>MPFVKGFEPISLRDTNLFEPIKIGNTQLAHRAVMPPLTRMRATHPGNIPNKEWAAVYYGQRAQRPGTMIITEGTFISPQAGGYDNAPGIWSDEQVAEWKNIFLAIHDCQSFAWVQLWSLGWASFPDVLARDGLRYDCASDRVYMNATLQEKAKDANNLEHSLTKDDIKQYIKDYIHAAKNSIAAGADGVEIHSANGYLLNQFLDPHSNKRTDEYGGTIENRARFTLEVVDALIETIGPERVGLRLSPYGTFNSMSGGAEPGIIAQYSYVLGELEKRAKAGKRLAFVHLVEPRVTDPSLVEGEGEYSEGTNDFAYSIWKGPIIRAGNYALHPEVVREQVKDPRTLIGYGRFFISNPDLVYRLEEGLPL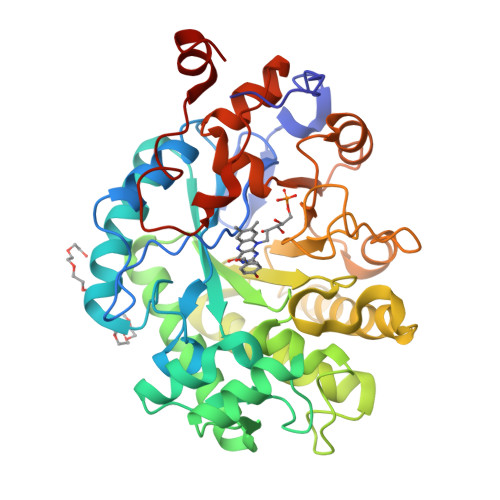NKYDRSTFYTMSAEGYTDYPTYEEAVDLGWNKN[2x]>[4x]MGSSHHHHHHSSGSAAYHIDEEVGFALPNPQENLPDFYNDWMFIAKHLPDLIESGQLRERVEKLNMLSIDHLTDHKSQRLARLVLGCITMAYVWGKGHGDVRKVLPRNIAVPYCQLSAALELPPILVYADCVLANWKKKDPNKPLTYENMDVLFSFRDGDCSKGFFLVSLLVEIAAASAIKVIPTVFKAMQMQERDTLLKALLEIASCLEKALQVFHQIHDHVNPKAF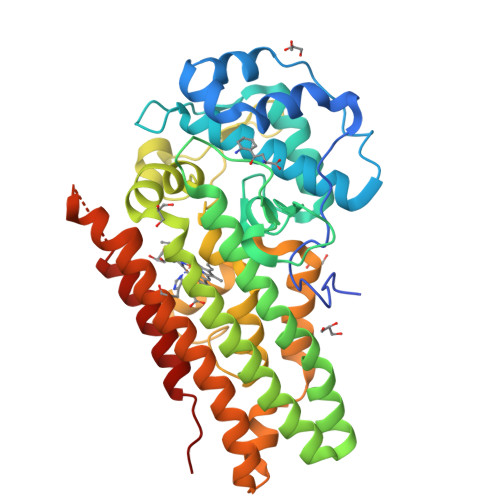FSVLRIYLSGWKGNPQLSDGLVYEGFWEDPKEFAGGSAGQSSVFQCFDVLLGIQQTAGGGHAAQFLQDMRRYMPPAHRNFLCSLESNPSVREFVLSKGDAGLREAYDACVKALVSLRSYHLQIVTKYILIPASQQPKENKTSEDPSKLEAKGTGGTDLMNFLKTVRSTTEKSLLKEG2-(acetylamido)-2-deoxy-D-glucono-1,5-lactone | C8 H13 N O6 | 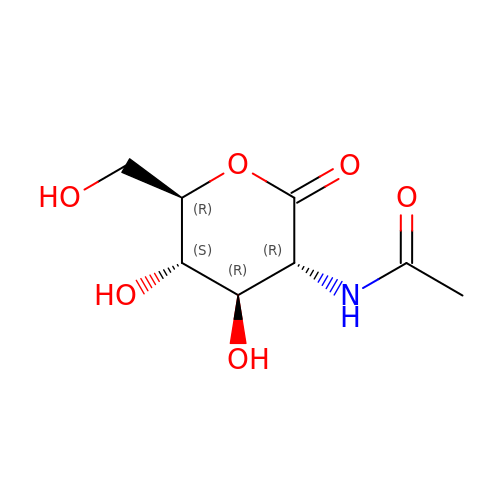NELQYZRSPDCGRQ-DBRKOABJSA-N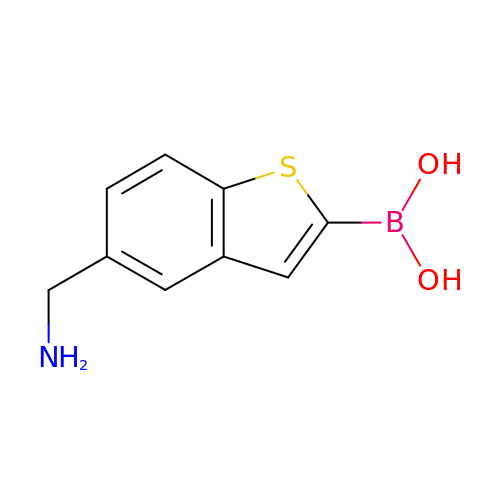[5-(aminomethyl)-1-benzothiophen-2-yl]boronic acid | C9 H10 B N O2 S | AMRAXCBFZWIMEQ-UHFFFAOYSA-N>MTVSASKTAQQLKYIKDSIKTIPDYPKAGILFRDVTSLLENPKAYSASIELLSEHYSESGVTKVVGTEARGFLFGAPVALALGVGFVPVRKPGKLPRETISESYELEYGTDTLEIHTDSIQPGDKVL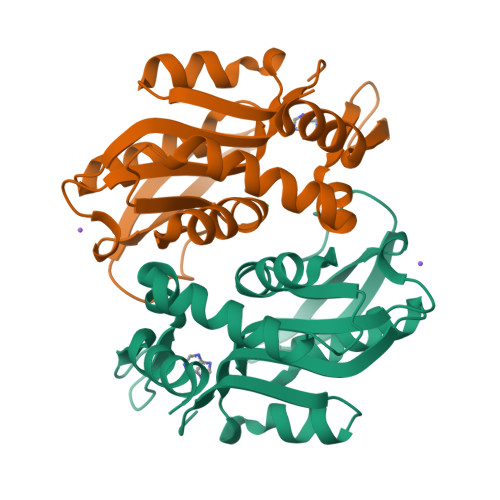VVDDLLATGGTIEATVKLIRRLGGEVVHAAFIINLPELGGEARLTQQGIHCYSLVSFDGH[2x]>[2x]GSNLTSAPVPSTTTRSLTACPEESPLLVGPMLIEFNIPVDLKLIEQQNPKVKLGGRYTPMDCISPHKVAIIIPFRNRQEHLKYWLYYLHPILQRQQLDYGIYVINQAGESMFNRAKLLNVGFKEALKDYDYNCFVFSDVDLIPMNDHNTYRCFSQPRHISVAM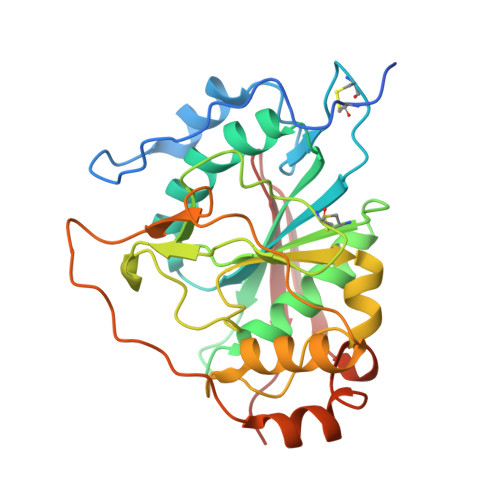DKFGFSLPYVQYFGGVSALSKQQFLSINGFPNNYWGWGGEDDDIYNRLAFRGMSVSRPNAVIGKCRMIRHSRDKKNEPNPQRFDRIAHTKETMLSDGLNSLTYMVLEVQRYPLYTKITVDIGTPS>[2x]SNAMKHIHIIGIGGTFMGGLAAIAKEAGFEVSGCDAKMYPPMSTQLEALGIDVYEGFDAAQLDEFKADVYVIGNVAKRGMDVVEAILNLGLPYISGPQWLSENVLHHHWVLGVAGTHGKTTTASMLAWVLEYAGLAPGFLIGGVPENFGVSARLPQTPRQDPNS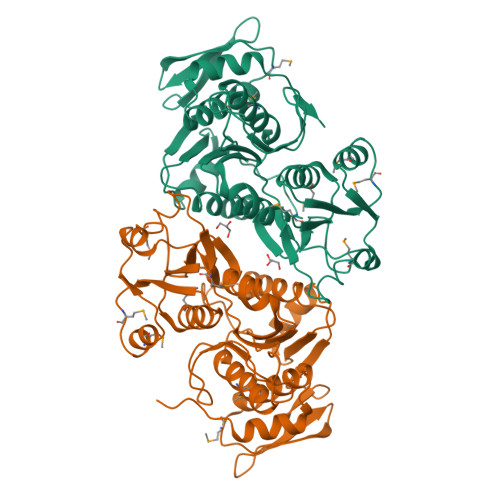QSPFFVIEADEYDTAFFDKRSKFVHYRPRTAVLNNLEFDHADIFADLGAIQTQFHYLVRTVPSEGLIVCNGRQQSLQDTLDKGCWTPVEKFGTEHGWQAGEANADGSFDVLLDGKTAGRVKWDLMGRHNRMNALAVIAAARHVGVDIQTACEALGAFKNVKR> GAGCAGACTTGACACCACTCA;> TGTCA;> TCTGAGTGA;> GGTCTGC

In this work, we exhaustively probe the ability of all 36 immobile HJ sequences to form DNA crystals in two different designed systems. Three separate self-assembling DNA crystal systems are described in this report: the “4 × 5” and “4 × 6” designs (collectively referred to as the 4 × N systems), and a third construct with a “scrambled” sequence variant of the 4 × 6 lattices. Self-assembly was mediated by three constituent oligonucleotides: (S1) containing four sequence repeats of either 5 or 6 bases; (S2) composed of 21 bases containing complementary regions to both (S1); and (S3) which forms the second junction crossover. The HJ serves as the fundamental component at the core of each unit, and the ultimate assembly of the full lattice is facilitated by the complementary 2-base sticky ends that tail each duplex.

Each asymmetric unit could be defined as either a HJ containing 10 and 11 bp on each arm, or as a 21-bp linear duplex. The 4 × 5 system robustly crystallized with 75% of the junctions, and we obtained crystals in all but 9 of 36 sequences. Of the resulting structures, 18 exhibited P32 symmetry with average cell dimensions a = b = 68.85 Å c = 60.09 Å, with only nine retaining the original P3221 symmetry with average cell edges a = b = 68.17 Å c = 60.60 Å. Although the cell parameters between the two symmetries were virtually indistinguishable, the differences between the periodicity of the lattices is dramatic, with vastly different cavity sizes.> SNAMFAPQGLAQFIKVNVTLENGEPVFIYTDANGQVCQGDITVTQAGTITYLLNDQTLKGLKFVGVGFVTPFDGIIDAVTIS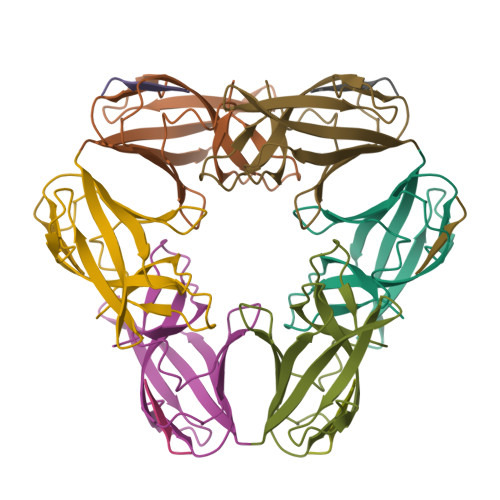SDGMLVQLVDLDKTPGTTKFQFVLSNTANTLLVLSAD;> PQIINRPQN> GSVPALWSEVNRYGQNGDFTRALKTVNKILQINKDDVTALHCKVVCLIQNGSFKEALNVINTHTKVLANNSLSFEKAY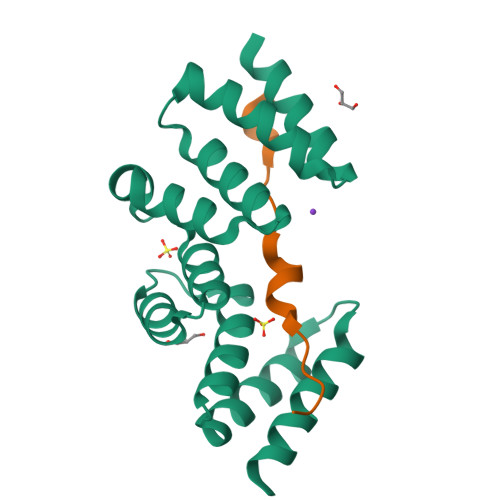CEYRLNRIENALKTIESANQQTDKLKELYGQVLYRLERYDECLAVYRDLVRNSQDDYDEERKTNLSAVVAAQSNWEKVVPGS;> MGSQVKDNKPLVERFETFCLDPSLVTKQANLVHFPPGFQPIPCKPLFFDLALNHVAFPPLEDKLEQKTKSG>GATESGKRMDCPALPPGWKKEEVIKKSGLSAGKSDVYYFSPSGKKFRSKPQLARYLG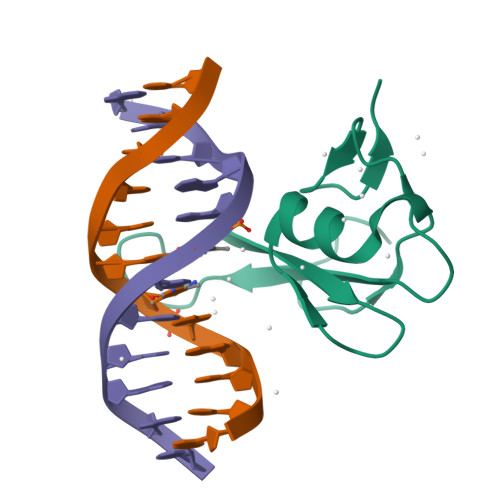NTVDLSSFDFRTGKMMPSKLQK[2x]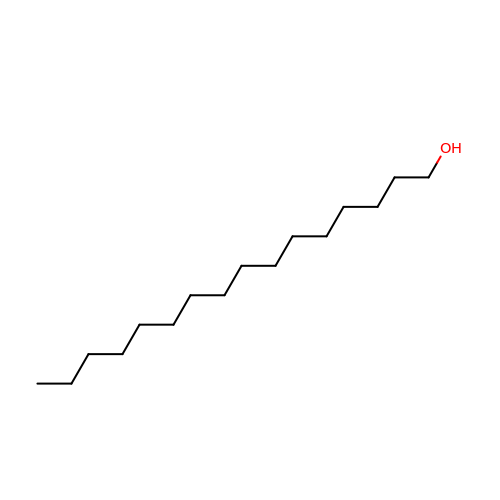HEXADECAN-1-OL | C16 H34 O | BXWNKGSJHAJOGX-UHFFFAOYSA-N>[2x]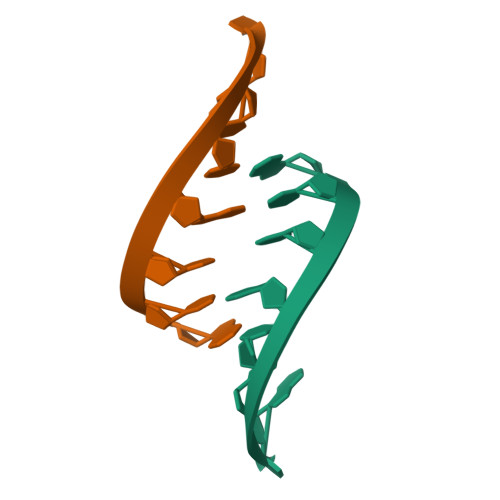GCCGCCGC>[5x]AMADYDTYVSNVQINNLSYGVYTSGGKETQFFCIGLKHGSEAISINAMCKVDVYGNHKQGFDNMLNTAKYYYTTGGDVRIYYKENVWRD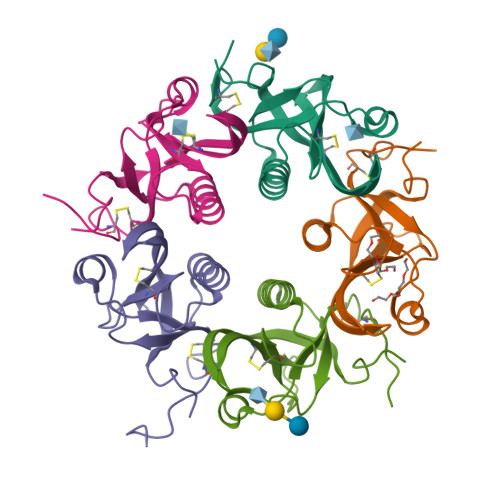PDFKSAFSSRELIAITTCSSSSYCMGPTVTNLESD> MNPADLSGLSGKELARARRAALSKQGKAAVSNKTASVNRSTKQAASSINTNQVRSSVNEVPTDYQMADQLCSTIDHADFGTESNRVRDLCRQRREALSTIGKKAVKTNGKPSGRVRPQQSVVHNDAMIENAGDTNQSSSTSLNNELSEICSIADDMPERFGSQAKTVRDICRARRQALSERGTRAVPPKPQSQGGPGRNGYQIDGYLDTALHGRDAAKRHREMLCQYGRGTAPSCKPTGRVKNSVQSGNAAPKKVETGHTLSGGSVTGTQVDRKSHVTGNEPGTCRAVTGTEYVGTEQFTSFCNTSPKPNATKVNVTTTARGRPVSGTEVSRTEKVTGNESGVCRNVTGTEYMSNEAHFSLCGTAAKPSQADKVMFGATARTHQVVSGSDEFRPSSVTGNESGAKRTITGSQYADEGLARLTINGAPAKVARTHTFAGSDVTGTEIGRSTRVTGDESGSCRSISGTEYLSNEQFQSFCDTKPQRSPFKVGQDRTNKGQSVTGNLVDRSELVTGNEPGSCSRVTGSQYGQSKICGGGVGKVRSMRTLRGTSVSGQQLDHAPKMSGDERGGCMPVTGNEYYGREHFEPFCTSTPEPEAQSTEQSLTCEGQIISGTSVDASDLVTGNEIGEQQLISGDAY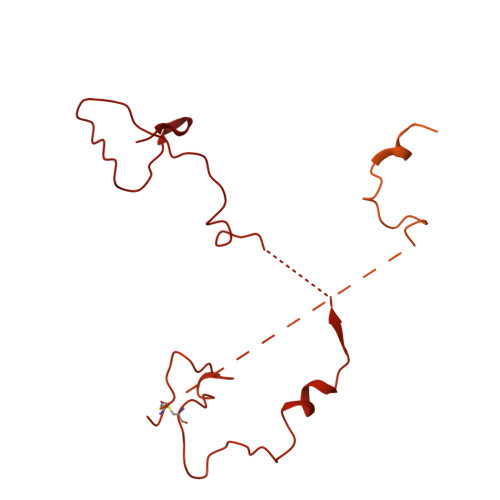VGAQQTGCLPTSPRFNQTGNVQSMGFKNTNQPEQNFAPGEVMPTDFSIQTPARSAQNRITGNDIAPSGRITGPGMLATGLITGTPEFRHAARELVGSPQPMAMAMANRNKAAQAPVVQPEVVATQEKPELVCAPRSDQMDRVSGEGKERCHITGDDWSVNKHITGTAGQWASGRNPSMRGNARVVETSAFANRNVPKPEKPGSKITGSSGNDTQGSLITYSGGARG~{N}-(4-phenylazanylquinazolin-7-yl)ethanamide | 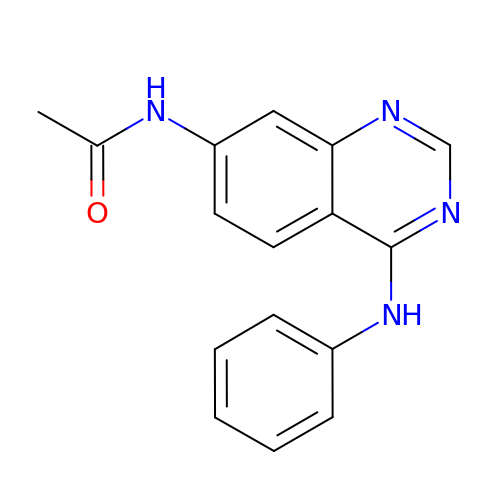C16 H14 N4 O | YGGWNWGVYREPPF-UHFFFAOYSA-N> MNQIDAHKLTIILRDATERLTFLDTINRQDDLSSELAGYEISKLLKKQKNLENQYADLVQLRTSLTGIQNKKNLIETQTKIVDVAQNLKESTKKLCRLFKENPDLESDALKVKKDRIQFMAVIEQLIQMVQNNSLTKFQSMTTLELEDQDRLRKLIFREKELYQEIKKLQFDRNQENKEYDNEQKDTNLKIQNLKERLLYKKARAQLK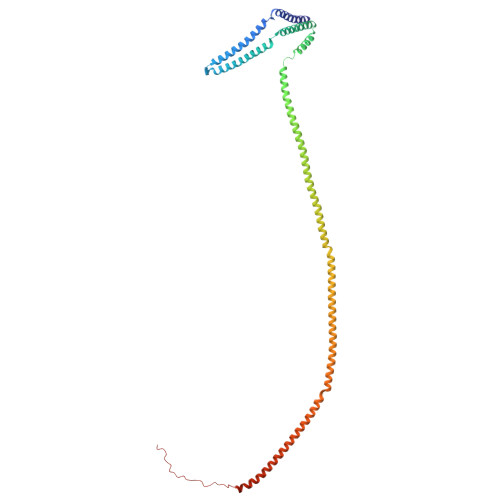NQYKEKEARAEEGTQQRMYEFEQKQLKEKINNLKQKTDTENMVHEQLRNFLIEKEDQIKQKSDEWAKKVETCREQLQEEIDRLTVEKEKKQEELRELRERDQKEQEEKDRRERQELEEADRKQQEELDQIRLDNAIKLIQIEYQEWKDAGGGKKKRKKGKKKKK> XXXXXXXXXXXXXXXXXXXXXXXXXXXXXXXXXXXXXXXXXXXXXXXXXXXXXXXXXXXXXXXXXXXXXXXXXXXXXXXXXXXXXXXXXXXXXXXXXXXXXXXXXXXXXXXXXXXXXXXXXXXXXXXXXXXXXXXXXXXXXXXXXXXXXXXXXXXXXXXXXXXXXXXXXXXXXXXXXXXXXXXXXXXXXXXXXXXXXXXXXXXXXXXXXXXXXXXXXXXXXXXXXXXXXXXXXXXXXXXXXXXXXXXXXXXXXXXXXXXXXXXXXXXXXXXXXXXXXXXXXXXXXXXXXXXXXXXXXXXXXXXXXXFSTNFRDTVDILVGWHIDHTQKPSLTQQVSGWLQSLEPFWVADLAFSTTLLGQFLEDMEAYAEDLSHVASGESVDEDVPPPSVSLPKLAALLRVFSTVVRSIGERFSPIRGPPITEAYVTDVLYRVMRCVTAANQVFFSEAVLTAANECVGVLLGSLDPSMTIHCDMVITYGLDQLENCQTCGTDYIISVLNLLTLIVEQINTKLPSSFVEKLFIPSSKLLFLRYHKEKEVVAVAHAVYQAVLSLKNIPVLETAYKLILGEMTCALNNLLHSLQLPEACSEIKHEAFKNHVFNVDNAKFVVIFDLSALTTIGNAKNSLIGMWALSPTVFALLSKNLMIVHSDLAVHFPAIQYAVLYTLYSHCTRHDHFISSSLSSSSPSLFDGAVISTVTTATKKHFSIILNLLGILLKKDNLNQDTRKLLMTWALEAAVLMRKSETYAPLFSLPSFHKFCKGLLANTLVEDVNICLQACSSLHALSSSLPDDLLQRCVDVCRVQLVHSGTRIRQAFGKLLKSIPLDVVLSNNNHTEIQEISLALRSHMSKAPSNTFHPQDFSDVISFILYGNSHRTGKDNWLERLFYSCQRLDKRDQSTIPRNLLKTDAVLWQWAIWEAAQFTVLSKLRTPLGRAQDTFQTIEGIIRSLAAHTLNPDQDVSQWTTADNDEGHGNNQLRLVLLLQYLENLEKLMYNAYEGCANALTSPPKVIRTFFYTNRQTCQDWLTRIRLSIMRVGLLAGQPAVTVRHGFDLLTEMKTTSLSQGNELEVTIMMVVEALCELHCPEAIQGIAVWSSSIVGKNLLWINSVAQQAEGRFEKASVEYQEHLCAMTGVDCCISSFDKSVLTLANAGRNSASPKHSLNGESRKTVLSKPTDSSPEVINYLGNKACECYISIADWAAVQEWQNSIHDLKKSTSSTSLNLKADFNYIKSLSSFESGKFVECTEQLELLPGENINLLAGGSKEKIDMKKLLPNMLSPDPRELQKSIEVQLLRSSVCLATALNPIEQDQKWQSITENVVKYLKQTSRIAIGPLRLSTLTVSQSLPVLSTLQLYCSSALENTVSNRLSTEDCLIPLFSEALRSCKQHDVRPWMQALRYTMYQNQLLEKIKEQTVPIRSHLMELGLTAAKFARKRGNVSLATRLLAQCSEVQLGKTTTAQDLVQHFKKLSTQGQVDEKWGPELDIEKTKLLYTAGQSTHAMEMLSSCAISFCKSVKAEYAVAKSILTLAKWIQAEWKEISGQLKQVYRAQHQQNFTGLSTLSKNILTLIELPSVNTMEEEYPRIESESTVHIGVGEPDFILGQLYHLSSVQAPEVAKSWAALASWAYRWGRKVVDNASXXXXXXXXXXXXXXXXXXXXXXXXXXXXXXXXXXXXXXXXXXXXXXXXXXXXXXXXXXXXXXXXXXXXXXXXXXXXXXXXXXXXXXXXEGVIKVWRKVVDRIFSLYKLSCSAYFTFLKLNAGQIPLDEDDPRLHLSHRVEQSTDDMIVMATLRLLRLLVKHAGELRQYLEHGLETTPTAPWRGIIPQLFSRLNHPEVYVRQSICNLLCRVAQDSPHLILYPAIVGTISLSSESQASGNKFSTAIPTLLGNIQGEELLVSECEGGSPPASQDSNKDEPKSGLNEDQAMMQDCYSKIVDKLSSANPTMVLQVQMLVAELRRVTVLWDELWLGVLLQQHMYVLXXXXXXXXXXXXXXXXXXXXXXXXXXXXXXXXXXXXXXXXXXXXXXXXXXXXXXXXPHEKWFQDNYGDAIENALEKLKXXXXXXXXXXXXXXXXXXXXXXXXXXXXXXXYILRLEEISPWLAAMTNTEIALPGEVSARDTVTIHSVGGTITILPTKTKPKKLLFLGSDGKSYPYLFKGLEDLHLDERIMQFLSIVNTMFATINRQETPRFHARHYSVTPLGTRSGLIQWVDGATPLFGLYKRWQQREAALQAQKAQDSYQTPQNPGIVPRPSELYYSKIGPALKTVGLSLDVSRRDWPLHVMKAVLEELMEATPPNLLAKELWSSCTTPDEWWRVTQSYARSTAVMSMVGYIIGLGDRHLDNVLIDMTTGEVVHIDYNVCFEKGKSLRVPEKVPFRMTQNIETALGVTGVEGVFRLSCEQVLHIMRRGRETLLTLLEAFVYDPLVDWTAGGEAGFAGAVYGGGGQQAESKQSKREMEREITRSLFSSRVAEIKVNWFKNRDEMLVVLPKLDGSLDEYLSLQEQLTDVEKLQGKLLEEIEFLEGAEGVDHPSHTLQHRYSEHTQLQTQQRAVQEAIQVKLNEFEQWITHYQAAFNNLEATQLASLLQEISTQMDLGPPSYVPATAFLQNAGQAHLISQCEQLEGEVGALLQQRRSVLRGCLEQLHHYATVALQYPKAIFQKHRIEQWKTWMEELICNTTVERCQELYRKYEMQYAPQPPPTVCQFITATEMTLQRYAADINSRLIRQVERLKQEAVTVPVCEDQLKEIERCIKVFLHENGEEGSLSLASVIISALCTLTRRNLMMEGAASSAGEQLVDLTSRDGAWFLEELCSMSGNVTCLVQLLKQCHLVPQDLDIPNPMEASETVHLANGVYTSLQELNSNFRQIIFPEALRCLMKGEYTLESMLHELDGLIEQTTDGVPLQTLVESLQAYLRNAAMGLEEETHAHYIDVARLLHAQYGELIQPRNGSVDETPKMSAGQMLLVAFDGMFAQVETAFSLLVEKLNKMEIPIAWRKIDIIREARSTQVNFFDDDNHRQVLEEIFFLKRLQTIKEFFRLCGTFSKTLSGSSSLEDQNTVNGPVQIVNVKTLFRNSCFSEDQMAKPIKAFTADFVRQLLIGLPNQALGLTLCSFISALGVDIIAQVEAKDFGAESKVSVDDLCKKAVEHNIQIGKFSQLVMNRATVLASSYDTAWKKHDLVRRLETSISSCKTSLQRVQLHIAMFQWQHEDLLINRPQAMSVTPPPRSAILTSMKKKLHTLSQIETSIATVQEKLAALESSIEQRLKWAGGANPALAPVLQDFEATIAERRNLVLKESQRASQVTFLCSNIIHFESLRTRTAEALNLDAALFELIKRCQQMCSFASQFNSSVSELELRLLQRVDTGLEHPIGSSEWLLSAHKQLTQDMSTQRAIQTEKEQQIETVCETIQNLVDNIKTVLTGHNRQLGDVKHLLKAMAKDEEAALADGEDVPYENSVRQFLGEYKSWQDNIQTVLFTLVQAMGQVRSQEHVEMLQEITPTLKELKTQSQSIYNNLVSFASPLVTDATNECSSPTSSATYQPSFAAAVRSNTGQKTQPDVMSQNARKLIQKNLATSADTPPSTVPGTGKSVACSPKKAVRDPKTGKAVQERNSYAVSVWKRVKAKLEGRDVDPNRRMSVAEQVDYVIKEATNLDNLAQLYEGWTAWV;> MSESGHSQPGLYGIERRRRWKEPGSGGPQNLSGPGGRERDYIAPWERERRDASEETSTSVMQKTPIILSKPPAERSKQPPPPTAPAAPPAPAPLEKPIVLMKPREEGKGPVAVTGASTPEGTAPPPPAAPAPPKGEKEGQRPTQPVYQIQNRGMGTAAPAAMDPVVGQAKLLPPERMKHSIKLVDDQMNWCDSAIEYLLDQTDVLVVGVLGLQGTGKSMVMSLLSANTPEEDQRTYVFRAQSAEMKERGGNQTSGIDFFITQERIVFLDTQPILSPSILDHLINNDRKLPPEYNLPHTYVEMQSLQIAAFLFTVCHVVIVVQDWFTDLSLYRFLQTAEMVKPSTPSPSHESSSSSGSDEGTEYYPHLVFLQNKARREDFCPRKLRQMHLMIDQLMAHSHLRYKGTLSMLQCNVFPGLPPDFLDSEVNLFLVPFMDSEAESENPPRAGPGSSPLFSLLPGYRGHPSFQSLVSKLRSQVMSMARPQLSHTILTEKNWFHYAARIWDGVRKSSALAEYSRLLA

The PI3K-related kinase (PIKK) SMG1 monitors the progression of metazoan nonsense-mediated mRNA decay (NMD) by phosphorylating the RNA helicase UPF1. SMG1 is a member of the phosphatidylinositol-3-kinase-related kinase (PIKK) family, which also includes the ATM, ATR, DNA-PKc, and mTOR kinases. Despite the confounding name reflecting a possible evolutionary origin with a lipid kinase, and in retrospect the ability of some PIKK family members to bind inositol-6-phosphate, all active PIKKs are Ser-Thr protein kinases. These large, multidomain enzymes share an overall similar architecture: a C-terminal catalytic module (comprising the so-called FAT, kinase, and FATC domains) and an N-terminal α-solenoid (that typically serves as a protein-protein interaction module). SMG8 and SMG9 form an unusual G-domain heterodimer.

Within the cryo-EM data set collected on an SMG1-8-9 complex incubated with SMG1i, we isolated a subset of particles missing any density for SMG8, hence representing an SMG1i-bound SMG1-9 complex. The corresponding 3.6 Å reconstruction not only showed a similar mode of interaction of SMG1i, but also several features distinct from SMG1 in isolation and the SMG1-8-9 ternary complex. Globally, the α-solenoid of SMG1 rearranges, consistent with the notion of a stepwise compaction of SMG1 upon binding first SMG9 and then SMG8 (Melero et al., 2014; Zhu et al., 2019). Locally, the mode of interaction between SMG9 and the SMG1 α-solenoid differs between the two complexes. In the binary SMG1-9 complex, the portion of SMG9 that interacts with the N-terminal HEAT repeat helices of SMG1 changes conformation, exploiting part of a binding site that was occupied by a short N-terminal segment of SMG8 in the ternary complex. Indeed, two hydrophobic residues of SMG9 (Leu456 and Leu457) take the place normally reserved for two hydrophobic residues of SMG8 (Leu351 and Leu352). Hence, the conformation of the SMG9 segment observed in the SMG1-9 complex is incompatible with the binding of SMG8 to this part of SMG1. Importantly, the reconstruction of SMG1-9 showed no ordered density at the active site for the PRD, which is in contrast to the ordered PRD density visualized in the SMG1i-bound SMG1-8-9 complex. The structure of an SMG1i-bound SMG1-9 complex reconstructed from the same data set as SMG1i-bound SMG1-8-9 did not show ordered density for the SMG1 PRD in the SMG1 active site. This suggested that an interaction between the SMG1 insertion and SMG8 was important for stabilizing the autoinhibited state of the complex.> RPVPMKRHIF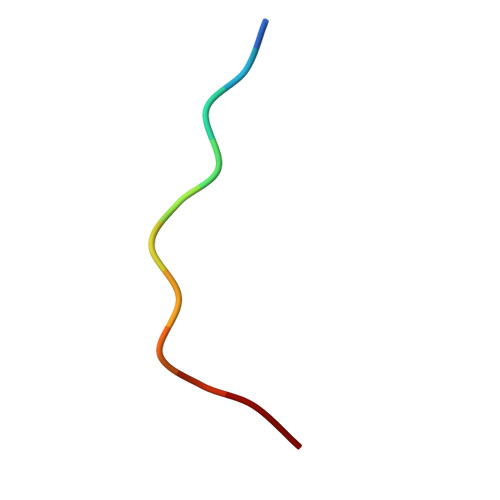R>MATETNYPVPYRSKLTEPFEPGQTLIIKGKTAEDSVRFTINLHNTSADFSGNDVPLHISVRFDEGKIVFNTFSKGEWGKEERKSNPYKKGDDIDIRIRAHDSKFSISVDQKEVKEYEHRVPLSSVTHFSVDGDILITYIHWGGKYYPVPYESGLAGDGLAPGKSLLIFATPEKKGKRFHINLLKKNGDIALHFNPRFDEKAIVRNSLISGEWGNEEREGKNPLEKGIGCDLEF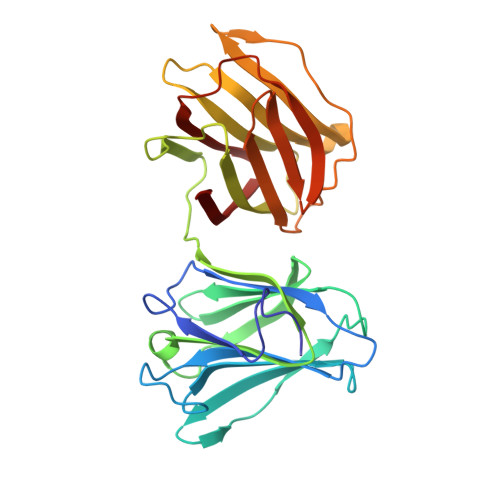RNEEYAFQIYVDGERFATYAHRLDPHDINGLQIGGDVEVTGIQMV[2x]> GSMKYKILKNLQFYYQENVIVVQINEKYLTNREHIFDVEESEQYFVDVEEI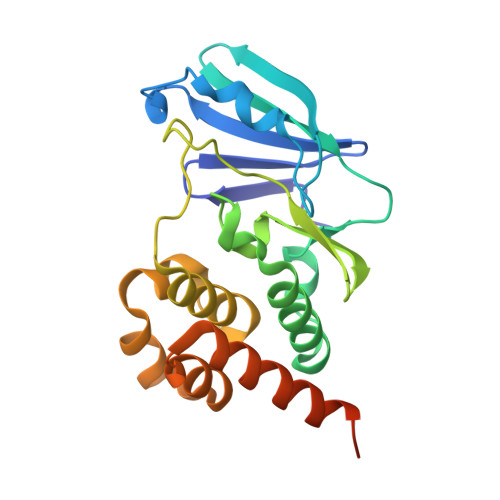LTKDGKLEIVYNRPNGYTPLLDLKEYADFYKLDIVNRLLEMNVLEKTNTYLAMQNILLKDTRDLLFIYKADHFDNLPYSTKEELEQWKNFICSFFGKFTLEKYEKNRIEVLTKEKNSFLNDVEAVESLESLRDLIKNRLTEEQKNFFSAELQDKKADVRKIRR> MSEFRIHHDVNELLSLLRVHGGDGAEVYIDLLQKNRTPYVTTTVSAHSAKVKIAEFSRTPEDFLKKYDELKSKNTRNLDPLVYLLSKLTEDKETLQYLQQNAKERAELAAAAVGSSTTSINVPAAASKISMQELEELRKQLGSVATGSTLQQSLELKRKMLRDKQNKKNSGQHLPIFPAWVYERPALIGDFLIGAGISTDTALPIGTLPLASQESAVVEDLLYVLVGVDGRYV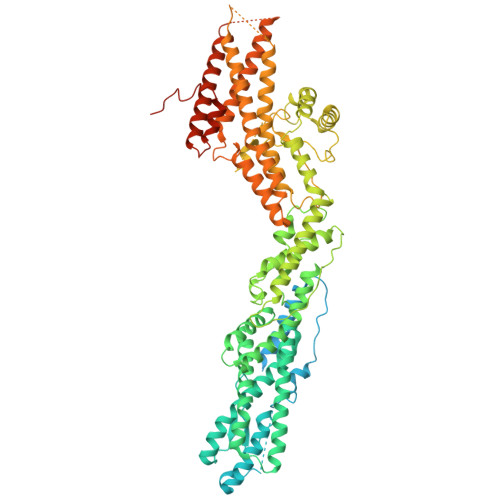SAQPLAGRQSRTFLVDPNLDLSIRELVHRILPVAASYSAVTRFIEEKSSFEYGQVNHALAAAMRTLVKEHLILVSQLEQLHRQGLLSLQKLWFYIQPAMRTMDILASLATSVDKGECLGGSTLSLLHDRSFSYTGDSQAQELCLYLTKAASAPYFEVLEKWIYRGIIHDPYSEFMVEEHELRKERIQEDYNDKYWDQRYTIVQQQIPSFLQKMADKILSTGKYLNVVRECGHDVTCPVAKEIIYTLKERAYVEQIEKAFNYASKVLLDFLMEEKELVAHLRSIKRYFLMDQGDFFVHFMDLAEEELRKPVEDITPPRLEALLELALRMSTANTDPFKDDLKIDLMPHDLITQLLRVLAIETKQEKAMAHADPTELALSGLEAFSFDYIVKWPLSLIINRKALTRYQMLFRHMFYCKHVERQLCSVWISNKTAKQHSLHSAQWFAGAFTLRQRMLNFVQNIQYYMMFEVMEPTWHILEKNLKSASNIDDVLGHHTGFLDTCLKDCMLTNPELLKVFSKLMSVCVMFTNCMQKFTQSMKLDGELGGQTLEHSTVLGLPAGAEERARKELARKHLAEHADTVQLVSGFEATINKFDKNFSAHLLDLLARLSIYSTSDCEHGMASVISRLDFNGFYTERLERLSAERSQKATPQVPVLRGPPAPAPRVAVTAQ>[6x]MGSSHHHHHHSSGLVPRGSGSDPTRKQKVEAQKQAEKLMKQIGVKNVKLSEYEMSIAAHLVDPLNMHVTWSDIAGLDDVITDLKDTVILPIKKKHLFENSRLLQPPKGVLLYGPPGCGKTLIAKATAKEAGCRFINLQPSTLTDKWYGESQKLAAAVFSLAIKLQPSIIFIDQID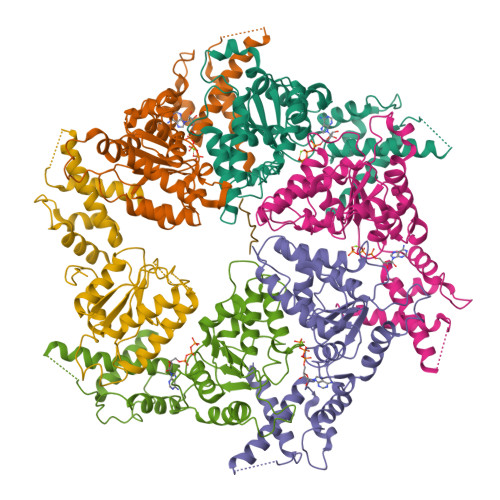SFLRNRSSSDHEATAMMKAQFMSLWDGLDTDHSCQVIVMGATNRPQDLDSAIMRRMPTRFHINQPALKQREAILKLILKNENVDRHVDLLEVAQETDGFSGSDLKEMCRDAALLCVREYVNSTSEESHDEDEIRPVQQQDLHRAIEKMKKSKDAAFQNVLTHVCLD> GPGSKSSISSISGRDDLMDYHRRQREERLREQEMERLERQRLETILSLCAEYTKPDSRLSTGTTVEDVQK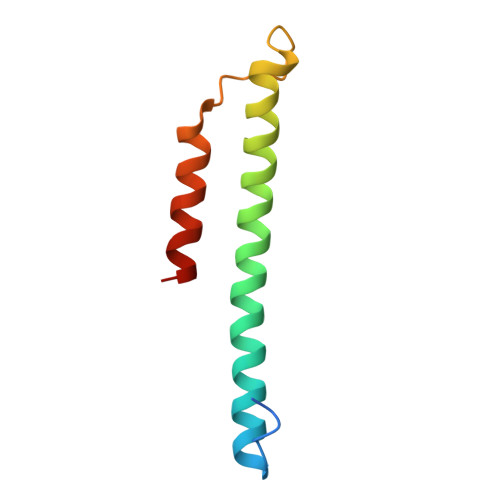INKELEKLQLSD> GPGPEIVDTCSLASPASVCRTKHLHLRCSVDFTRRTLTGTAALTVQSQEDNLRSLVLDTKDLTIEKVVINGQEVKYALGERQSYKGSPMEISLPIALSKNQEIVIEISFETSPKSSALQWLTPEQTSGKEHPYLFSQCQAIHCRAILPCQDTPSVKLTYTAEVSVPKELVALMSAIRDGETPDPEDPSRKIYKFIQKVPIPCYLIALVVGALESRQIGPRTLVWSEKEQVEKSAYEFSETESMLKIAEDLGGPYVWGQYDLLVLPPSFPYGGMENPCLTFVTPTLLAGDKSLSNVIAHEISHSWTGNLVTNKTWDHFWLNEGHTVYLERHICGRLFGEKFRHFNALGGWGELQNSVKTFGETHPFTKLVVDLTDIDPDVAYSSVPYEKGFALLFYLEQLLGGPEIFLGFLKAYVEKFSYKSITTDDWKDFLYSYFKDKVDVLNQVDWNAWLYSPGLPPIKPNYDMTLTNACIALSQRWITAKEDDLNSFNATDLKDLSSHQLNEFLAQTLQRAPLPLGHIKRMQEVYNFNAINNSEIRFRWLRLCIQSKWEDAIPLALKMATEQGRMKFTRPLFKDLAAFDKSHDQAVRTYQEHKASMHPVTAMLVGKDLKVD

LTA4H catalyzes the final and rate limiting step in the biosynthesis of pro-inflammatory LTB4, that is, the vinylogous hydrolysis of the epoxide, LTA4. LTA4 binds to a deep L-shaped hydrophobic channel which forms one of two lobes of the catalytic site of the enzyme. The second lobe of the catalytic site of LTA4H is a more open and hydrophilic pocket, and forms the aminopeptidase activity of the enzyme. While less is known about the physiological relevance of the aminopeptidase activity of LTA4H, Snelgrove and co-workers suggested that it can degrade the tripeptide PGP which has been reported to be a collagen-derived matrikine and neutrophil chemoattractant.

As the unbiased approach did not yield a compound sparing the aminopeptidase activity, we decided to test whether we could obtain a potent aminopeptidase-sparing inhibitor by truncating an optimized LTA4H inhibitor, JNJ-2699313518, with the hypothesis that the potency against the epoxide hydrolase activity was not strictly coupled to potency against the aminopeptidase activity. Overlaying the structure of LTA4H bound JNJ-26993135 (compound 11) to that of PGP bound in the active site showed that simultaneous binding of the two ligands would not be possible due to steric effects. However, we hypothesized that by removing the part of the compound which interacts with the Zn2+, we would be able to have simultaneous binding of the PGP and the truncated compound to LTA4H. Removing the carboxylic acid group of JNJ-26993135 led to a compound that was still a potent epoxide hydrolase inhibitor (compound 12), but also did not spare the aminopeptidase activity. Replacement of the piperidine-4 carboxylic acid by only a carboxylic acid moiety, led to a compound inactive in both assays (compound 13). Since most reported LTA4H inhibitors extend from the hydrophobic pocket into the aminopeptidase binding site, they do not exhibit any epoxide hydrolase specificity.>[12x]DEL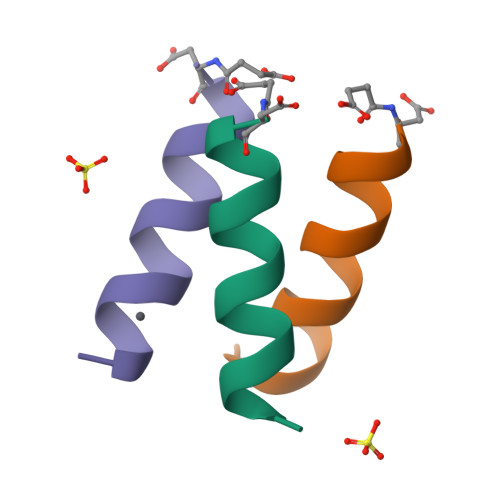ERRIRELEARIK> MSIVMQLQDVAESTRLGPLSGEVRAGEILHLVGPNGAGKSTLLARMAGMTSGKGSIQFAGQPLEAWSATKL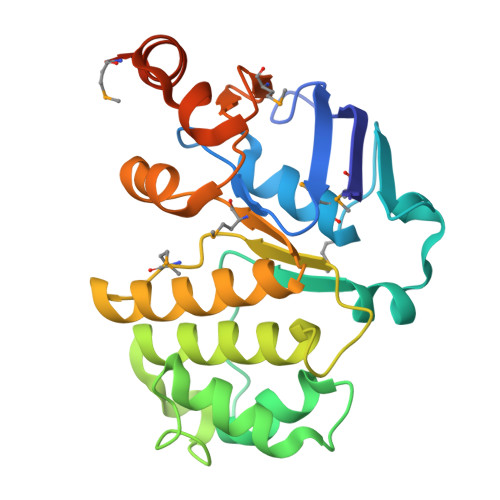ALHRAYLSQQQTPPFATPVWHYLTLHQHDKTRTELLNDVAGALALDDKLGRSTNQLSGGEWQRVRLAAVVLQITPQANPAGQLLLLDEPMNSLDVAQQSALDKILSALCQQGLAIVMSSHDLNHTLRHAHRAWLLKGGKMLASGRREEVLTPPNLAQAYGMNFRRLDIEGHRMLISTI> MQSSVNEFLTPRHIDVQVVSQTRAKITLEPLERGFGHTLGNALRRILLSSMPGCAVVEAEIDGVLHEYSAIEGVQEDVIEILLNLKGLAIKLHGRDEVTLTLAKKGSGVVTAADIQLDHDVEIINGDHVIANLADNGALNMKLKVARGRGYEPADARQSDEDESRSIGRLQLDASFSPVRRVSYVVENARVEQRTNLDKLVLDLETNGTLDPEEAIRRAATILQQQLAAFVDLKGDSEPVVEEQEDEIDPILLRPVDDLELT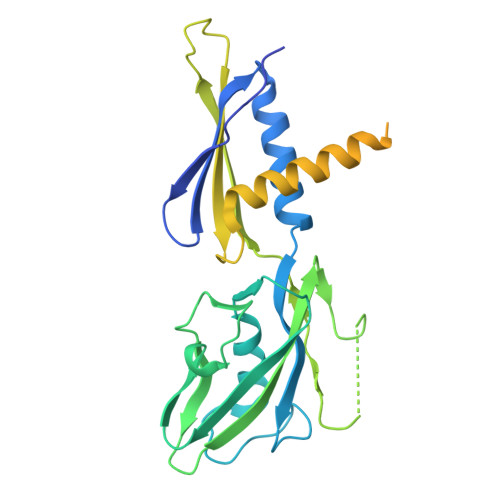VRSANCLKAENIYYIGDLIQRTEVELLKTPNLGKKSLTEIKDVLASRGLSLGMRLDNWPPASLKKDDKATA By performing a screen based on affinity purification and mass spectrometry, we observed that a previously uncharacterised phage protein specifically binds to two RNA binding sites within the CTH of RNase E, and by doing so efficiently inhibits the RNA binding and degradation activity of the degradosome assembly. We have determined the structure of this protein (termed Dip, ‘degradosome interacting protein’) by X-ray crystallography and show that it forms an open-clamp like homo-dimeric structure, and binding of Dip to RNA binding regions within RNase E is characterized functionally and structurally. As with the 756–775 binding site, 9S rRNA can be competitively displaced from the 583–636 fragment by Dip, and the addition of a 4-fold excess of Dip is able to completely remove the bound RNA from the RNase E fragment. These results demonstrate that Dip targets both RNA binding sites in the C-terminal half of the RNA degradosome, and consequently blocks the binding of RNA to the RNase E subunit.

The 2.2 Å structure of Dip reveals a clamp like homodimeric structure, with the dimeric architecture presenting a grooved, concave face resembling a partially opened scroll. The dimeric form was confirmed to be the predominant species in solution by analytical ultracentrifugation, while self-interaction was showed during a bacterial two-hybrid analyses (Data not shown). Interestingly, electron density for an unknown small molecule ligand can be seen in this region in the structure of apo-Dip, which we have modelled as a single arginine amino acid. The unique structure of this protein resembles a partially opened scroll or a clamp, and it is tempting to imagine that the two protomers of Dip could act as pincers to capture a binding partner at the dimer interface. However, through a combination of structural, biochemical and bioinformatics analyses we can conclude that the binding site for RNase E is actually on the outer surfaces of the Dip dimer, and not within the “clamp”. Since one dimer of Dip possesses two binding sites on its surface, several possible RNase E binding models can be envisaged.

>[2x]MTQFNITWEEQLQALSKLDGLHHPHKLEDISVHWVFNPVDISVFVTCATMSSHNTHYTFKPQSSPDDAMVREYVLSRIIADNLKYVDNLYLAAGAVICGNDEYISDGNVVGIHIADGVGGNKLILPVIEFMPGVHVDDISDKLIKSSSYQGIFKTDNLEEFEFLVDKKNANNVKELILAYTDYFANKLAFKDPAEPAVEMYQFIDRTEVYFSFEGCHPDVEEVLFTIKIVRYNQPLNSTAMQVFLKNPLLSHIRTVVRQDLPAKFVGGVLFNFKGHHHHHH2-(octanoylamino)benzoic acid | C15 H21 N O3 | 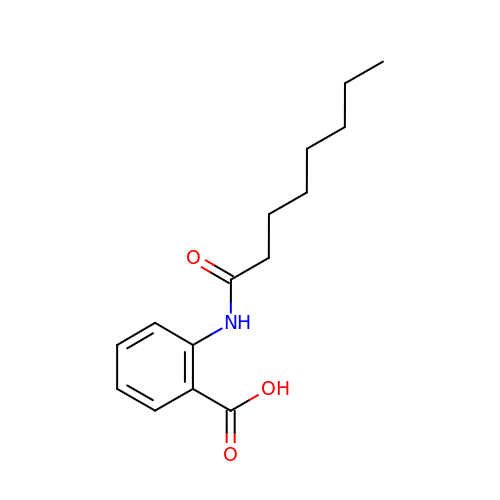DIBJPKPIMHBNDD-UHFFFAOYSA-N[2-(6-AMINO-9H-PURIN-9-YL)-1-METHYLETHOXY]METHYL-TRIPHOSPHATE | C9 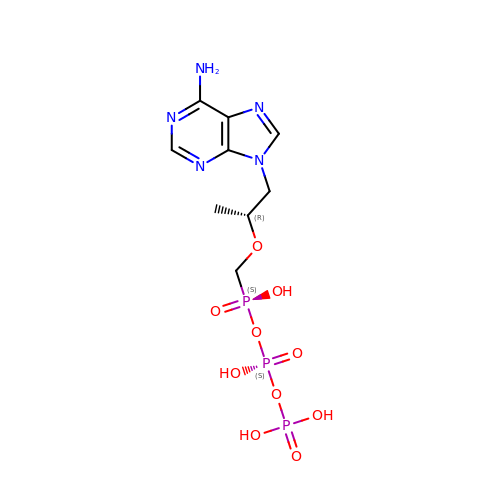H16 N5 O10 P3 | IACQCQDWSIQSRP-ZCFIWIBFSA-N> SDNAIAMEAAHSKSTEECLAYFGVSETTGLTPDQVKRHLEKYGHNELPAEEGKSLWELVIEQFEDLLVRILLLAACISFVLAWFEEGEETITAFVEPFVILLILIANAIVGVWQERNAENAIEALKEYEPEMGKVYRADRKSVQRIKARDIVPGDIVEVAVGDKVPADIRILSIKSTTLRVDQSILTGESVSVIKHTEPVPDPRAVNQDKKNMLFSGTNIAAGKALGIVATTGVSTEIGKIRDQMAATEQDKTPLQQKLDEFGEQLSKVISLICVAVWLINIGHFNDPVHGGSWIRGAIYYFKIAVALAVAAIPEGLPAVITTCLALGTRRMAKKNAIVRSLPSVETLGCTSVICSDKTGTLTTNQMSVCKMFIIDKVDGDFCSLNEFSITGSTYAPEGEVLKNDKPIRSGQFDGLVELATICALCNDSSLDFNETKGVYEKVGEATETALTTLVEKMNVFNTEVRNLSKVERANACNSVIRQLMKKEFTLEFSRDRKSMSVYCSPAKSSRAAVGNKMFVKGAPEGVIDRCNYVRVGTTRVPMTGPVKEKILSVIKEWGTGRDTLRCLALATRDTPPKREEMVLDDSSRFMEYETDLTFVGVVGMLDPPRKEVMGSIQLCRDAGIRVIMITGDNKGTAIAICRRIGIFGENEEVADRAYTGREFDDLPLAEQREACRRACCFARVEPSHKSKIVEYLQSYDEITAMTGDGVNDAPALKKAEIGIAMGSGTAVAKTASEMVLADDNFSTIVAAVEEGRAIYNNMKQFIRYLISSNVGEVVCIFLTAALGLPEALIPVQLLWVNLVTDGLPATALGFNPPDLDIMDRPPRSPKEPLISGWLFFRYMAIGGYVGAATVGAAAWWFMYAEDGPGVTYHQLTHFMQCTEDHPHFEGLDCEIFEAPEPMTMALSVLVTIEMCNALNSLSENQSLMRMPPWVNIWLLGSICLSMSLHFLILYVDPLPMIFKLKALDLTQWLMVLKISLPV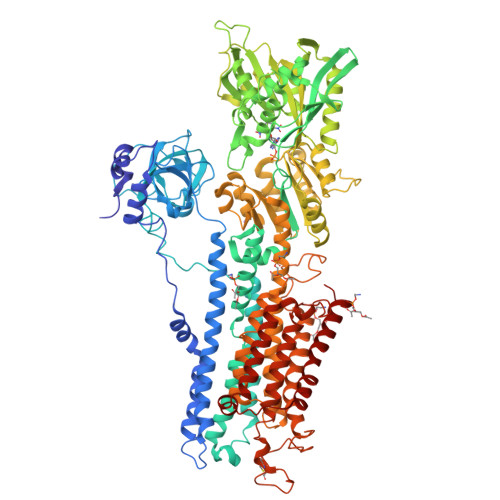IGLDEILKFIARNYLEG>EQEQQYDVHGNVISAAVYQKFHVYGPEDMVFDGDAGGLTIPGAGAFWGTLFTSDLQRLYKDTVSFQYNALGTYLNINFFDSSGGFLGHIQAGAVSAVV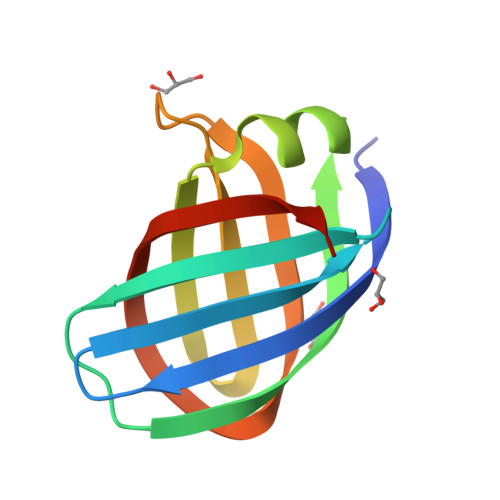GVGGGSGSWHNWEVA[2x]>[2x]MANKTYKIGKNAGYDGCGLCLAAISENEAIKVKYLRDICPDYDGDDKAEDWL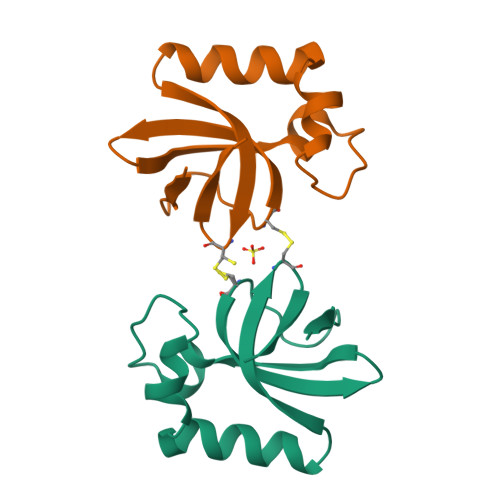RWGTDSRVKAAALEMEQYAYTSVGMASCWEFVEL[[(2~{S},3~{S},4~{R},5~{R})-5-(6-aminopurin-9-yl)-3,4-bis(oxidanyl)oxolan-2-yl]methoxy-oxidanyl-phosphoryl] 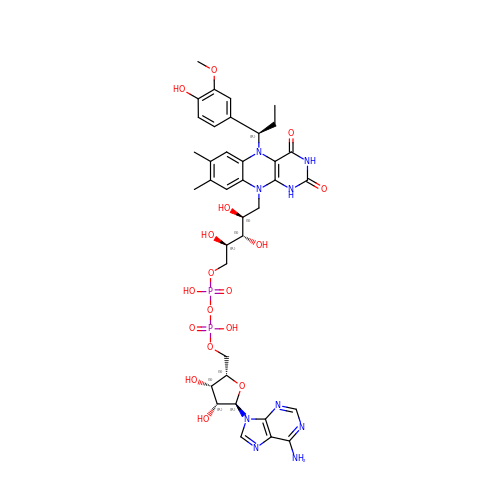[(2~{R},3~{S},4~{S})-5-[5-[(1~{R})-1-(3-methoxy-4-oxidanyl-phenyl)propyl]-7,8-dimethyl-2,4-bis(oxidanylidene)-1~{H}-benzo[g]pteridin-10-yl]-2,3,4-tris(oxidanyl)pentyl] hydrogen phosphate | C37 H47 N9 O17 P2 | VAUBFXXAVOWJEY-LKEIEZFZSA-N>[6x]SNAMKENKLDYIPEPMDLSLVDLPESLIQLSERIAENVHEVWAKARI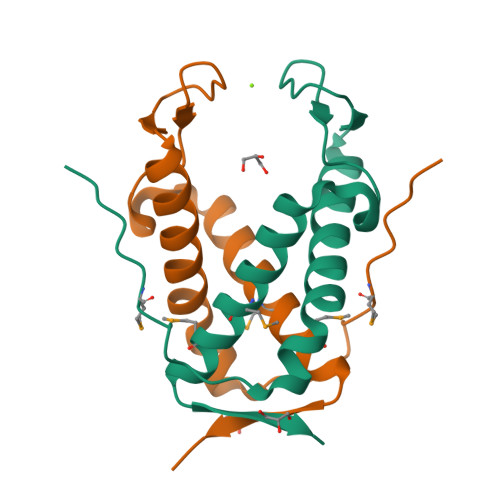DEGWTYGEKRDDIHKKHPCLVPYDELPEEEKEYDRNTAMNTIKMVKKLGFRIEKED> MAAERVFISPAKYVQGKNVITKIANYLEGIGNKTVVIADEIVWKIAGHTIVNELKKGNIAAEEVVFSGEASRNEVERIANIARKAEAAIVIGVGGGKTLDTAKAVADELDAYIVIVPTAASTDAPTSALSVIYSDDGVFESYRFYKKNPDLVLVDTKIIANAPPRLLASGIADALATWVEARSVIKSGGKTMAGGIPTIAAEAIAEKCEQTLFKYGKLAYESVKAKVVTPALEAVVEANTLLSGLGFESGGLAAAHAIHNGFTALEGEIHHLTHGEKVAFGTLVQLALEEHS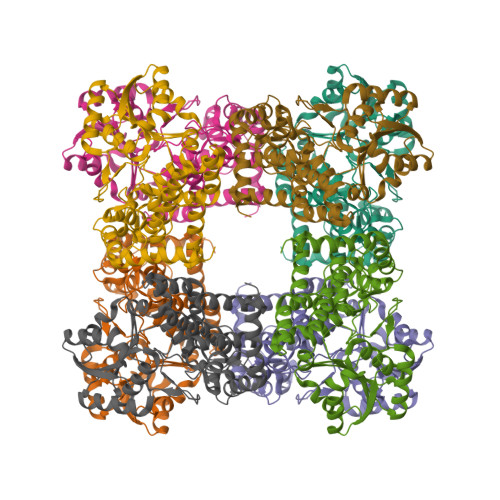QQEIERYIELYLCLDLPVTLEDIKLKDASREDILKVAKAATAEGETIHNAFNVTADDVADAIFAADQYAKAYKEKHRK Under conditions of sulphur limitation and in the presence of the inducer, N-acetylserine, CysB binds to cys promoters and activates the transcription of the downstream coding sequences. CysB is a homotetramer of 36 kDa subunits, each comprising a smaller N-terminal DNA binding domain and a C-terminal effector binding domain. CysB is a member of the LysR-type transcriptional regulator (LTTR) family, named after its founding member. To elucidate the subunit arrangement in the tetramer, we determined the crystal structure of intact CysB in complex with N-acetylserine.

The H32 and H3 crystal structures have 2 and 8 molecules in the asymmetric unit respectively. In the H32 crystal form, a crystallographic twofold axis of symmetry generates the CysB tetramer while the asymmetric unit of the H3 crystal form contains two CysB tetramers. There are two protomer types in each tetramer distinguished by the juxtaposition of the DNA binding and the effector binding domains. CysB(1–324) was crystallised in the presence of 10 mM of the inducer N-acetylserine. The ligand is enclosed in the prominent cleft between EBDI and EBDII. It is generally well defined in the electron density maps of all of the subunits across the two crystal forms though the occupancy is lower in the B molecule of the H32 crystal form. The carbonyl oxygen of the N-acetyl group of the ligand accepts hydrogen bonds from the hydroxyl of Thr100 and the amide –NH2 of Gln103. The side chain of the serine forms a charge-dipole interaction with the Glu150 carboxylate and a dipole–dipole interaction with the hydroxyl of Thr149. Meanwhile, the carboxylate of the ligand forms interactions with the phenolic hydroxyl of Tyr197, the aliphatic hydroxyls of Thr100 and Thr102 and an ordered water molecule.

>[2x]MKLQQLRYIVEVVNHNLNVSSTAEGLYTSQPGISKQVRMLEDELGIQIFARSGKHLTQVTPAGQEIIRIAREVLSKVDAIKSVAGEHTWPDKGSLYVATTHTQARYALPGVIKGFIERYPRVSLHMHQGSPTQIAEAVSKGNADFAIATEALHLYDDLVMLPCYHWNRSIVVTPEHPLATKGSVSIEELAQYPLVTYTFGFTGRSELDTAFNRAGLTPRIVFTATDADVIKTYVRLGLGVGVIASMAVDPVSDPDLVKLDANGIFSHSTTKIGFRRSTFLRSYMYDFIQRFAPHLTRDVVDTAVALRSNEDIEAMFKDIKLPEK> 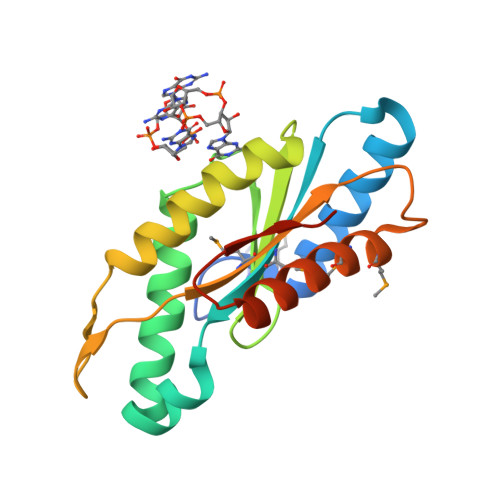MEQLAKLSMTDRLTGLLNRGTWENLVDAEYERFRRYGQATSLVMFDIDHFKPVNDTYGHLAGDEVIRHTADVTRNNIRQSDSAGRYGGEEFGIILPETDAESARVICERIREAIEKSTVSTSAGDIQYTVSMGIAQLTETPENYMQWMQKADEALYKAKESGRNKVVVSLEHHHHHH>GSSGSSGMKNIESLFDYSAGQFEFIDHLLTMGVGVHFAALIFFLVVSQFVAPKYRIATALSCIVMVSAGLILNSQAVMWTDAYAYVDGSYQLQDLTFSNGYRYVNWMATIPCLLLQLLIVLNLKGKELFSTATWLILAAWGMIITGYVGQLYEVDDIAQLMIWGAVSTAFFVVMNWIVGTKIFKNRATMLGGTDSTITKVFWLMMFAWTLYPIAYLVPAFMNNADGVVLRQLLFTIADISSKVIYGLMITYIAIQQ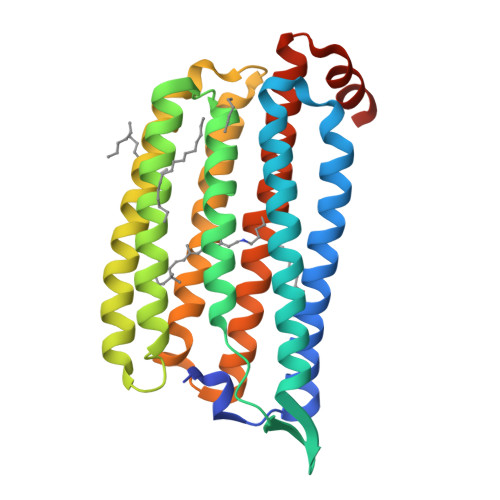SAAAGYVPAQQALGRIGMDSKAA[3x]The HDAC domains of class IIa HDACs repress the respective target genes by interacting with the C-terminal region of the silencing mediator for retinoid and thyroid receptor (SMRT) repression domain 3 (SRD3c). Here, we found that two conserved GSI-containing motifs of SRD3c are critical for HDAC4 binding. Two SMRT peptides including these motifs commonly form a β-hairpin structure in the cleft and block the catalytic entry site of HDAC4. They interact mainly with class IIa HDAC-specific residues of HDAC4 in a closed conformation.

For the SRD3c protein, we designed two peptides (SP1: −3HIRGSITQGIPRSYV+12, SP2: −2KEGSITQGTPLKY+11), which include the GSI motif in the sequences. For kinetic analysis of peptide binding to HDAC4c H976Y (R651-T1055), we performed ITC experiments and obtained a dissociation constant of 2.23 μM for SP1 and 18.8 μM for SP2. Overall, the refined HDAC4c-peptide structures superpose well on the apo-form structure, indicating that peptides binding did not rearrange the catalytic and structural zinc ion-binding sites. The bound peptides commonly form a β-hairpin structure of two β-strands in the HDAC4c cleft leading to the catalytic zinc ion. The hydrophobic I+3 residues (I1363 or I1459) are at the β-turn near the catalytic zinc ion and intervened with F812 and F871 at the end of the cleft and entrance to the catalytic pocket of the HDAC4c. At the two loops of S744–W762 and H803–G811 of the structural zinc ion-binding site, D759 hydrogen-bonds with the hydroxyl group of T+4 and peptidyl nitrogen atom between S+2 and I+3 in two peptides. Notably, D757 interacts indirectly with R+9 of the bound SP1 via a water molecule (w8), which is missing in the SP2-bound structure with L+9 at the corresponding position. According to the determined structures, the SP1 R+9 residue interacts with the structural zinc-binding region (although this interaction is water-mediated), and SP1 I+7 and SP2 T+7 are exposed to solvent without interacting with the protein, suggesting the greater importance of the SM1 R+9 residue than the I+7 residue. Interestingly, HDAC-binding activity was significantly decreased in the SM1 R+9L mutant (SM2 mimic), whereas the SM2 L+9R mutant (SM1 mimic) exhibited increased binding activity. The reverse SM2 mutant, an SM1-mimic L+9R mutant, showed increased binding activity to HDACs, which was comparable to that of wild-type SM1. These results suggest that formation of a β-hairpin structure along with an R+9 residue at the end of the second β-strand in SP1 is a major contributor to the SRD3c interaction with HDAC4c/-5c/-7c.

> HIRGSITQGIPRSY;> AFTTGLVYDTLMLKHQCTCGSSSSHPEHAGRIQSIWSRLQETGLRGKCECIRGRKATLEELQTVHSEAHTLLYGTNPLNRQKLDSKKLLGSLASVFVRLPCGGVGVDSDTIWNEVHSAGAARLAVGCVVELVFKVATGELKNGFAVVRPPGHHAEESTPMGFCYFNSVAVAAKLLQQRLSVSKILIVDWDVHHGNGTQQAFYSDPSVLYMSLHRYDDGNFFPGSGAPDEVGTGPGVGFNVNMAFTGGLDPPMGDAEYLAAFRTVVMPIASEFAPDVVLVSSGFDAVEGHPTPLGGYNLSARCFGYLTKQLMGLAGGRIVLALEGGYDLTAICDASEACVSALLGNELDPLPEKVLQQRPNANAVRSMEKVMEIHSKYWRCLQRTTSTAGRSLIEAQTCENEEA> SSQIRQNYSTEVEAAVNRLVNLYLRASYTYLSLGFYFDRDDVALEGVCHFFRQLAQQKMQGAERLLKMQNQRGGRALFQDLQKPSQDEWG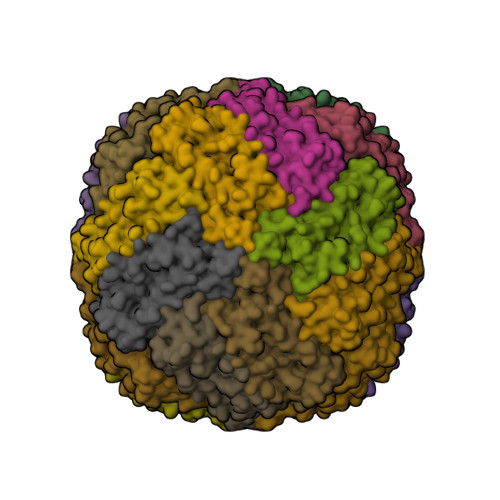TTPDAMKAAIVLEKSLNQALLDLHALGSAQADPHLCDFLESHFLDEEVKLIKKMGDHLTNIQRLVGSQAGLGEYLFERLTLKHD> GTQRVVQKRRHQMRILHPAQTAYVPVEQRPPPIPHSLTASSTVKRLLNNNTVAAKEAAKRINWGAYISHQRGVRWHPQGAWRVQFSRR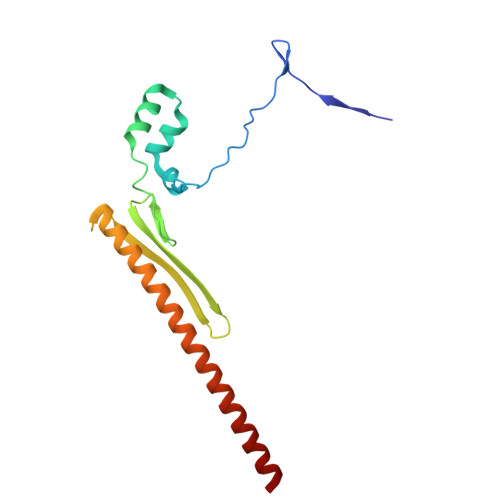NHERNFFVRCECYFRVGTYGFQMAKDLAIRYRQRLEKEWEELQEQWTKLDILEAEQRAKYKEKREEHLLL> GSVADIQQLEEKVDESDVRIYFNEKSSGGKISIDNASYNARKLGLAPSSIDEKKIKELYGDNLTYEQYLEYLSICVHDKDNVEELIKMFAHFDNNCTGYLTKSQMKNILTTWGDALTDQEAIDALNAFSSEDNIDYKLFCEDILQ;> GSLLRVQAHIRKKMV

We sought to employ a fragment-based approach toward targeting the interaction between the C-terminal “tail” of Plasmodium falciparum myosin A (PfmyoA) and binding partner myoA tail domain interacting protein (PfMTIP). This PPI is thought to be central to the malaria parasite’s ability to glide and invade host cells in a defined, directional manner, as correct localization of the myoA motor protein depends on its interaction with MTIP (called myosin light chain 1, MLC1, in other apicomplexan parasites such as Toxoplasma gondii). We and others have developed peptidic inhibitors of the PfMTIP–myoA complex by mimicking the C-terminal tail of myoA, which adopts a helical conformation and is “clamped” by two domains of MTIP (N- and C-terminal domains, NTD and CTD), burying >2000 Å2 of solvent-exposed protein surface upon complex formation. We have taken a different approach by studying isotopically labeled PfMTIPΔ60 (containing both MTIP domains) in solution using multidimensional NMR techniques, and recently reported assignments of the 1H,15N-HSQC spectra of both the “free” and “bound” states, along with a detailed analysis of the conformational dynamics and thermodynamics of the system. It was found that the free protein is highly flexible on a range of timescales from millisecond to sub-nanosecond exchange processes, which may explain the difficulty in crystallizing the protein in isolation.

The CSPs of 8 localized to the MTIP CTD including several contiguous MTIP–myoA hotspots, for example, Leu 168, Trp 171, Gly 172, Asp 173, Ala 174, and Thr 176 that form the loop connecting helices α6 and α7, involved in the key intramolecular clamp with Ser 108. Taken together, these results suggest that the primary amine linked to the furan via a thioether represent key features of 8. However, given that one end of the molecule was not necessary for interaction with MTIP, it was hypothesized that attachment of the key moieties of 8 to a myoA tail peptide would enable an X-ray structure of the bound fragment to be obtained. Because the N-terminal part of PfmyoA(799–818) binds to the same site as the fragment, we systematically truncated the myoA tail at this end to create a library of chimeric molecules. Synthesis of the chimeras (chimera) was achieved via Fmoc-based solid-phase peptide synthesis, with a glycine spacer attached to the N terminus of each myoA sequence to permit flexibility in the orientation of the fragment. Three different myoA tail sequences were prepared (terminating at Leu 805, Leu 804, and Ser 803); by analysis of residue-specific CSPs caused by the fragment and the crystal structure of the wild-type complex with PfmyoA(799–818), it was rationalized that these positions should provide enough space for the fragment to adopt a binding conformation. Notably, the terminal free amine, identified as a key feature of 8, forms a salt bridge with the side chain of Asp 173.>[5x]MSLINTKIKPFKNQAFKNGEFIEITEKDTEGRWSVFFFYPADFTFVCPTELGDVADHYEELQKLGVDVYAVSTDTHFTHKAWHSSSETIAKIKYAMIGDPTGALTRNFDNM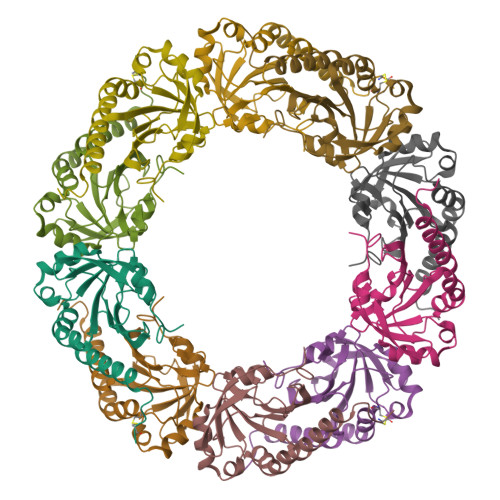REDEGLADRATFVVDPQGIIQAIEVTAEGIGRDASDLLRKIKAAQYVASHPGEVCPAKWKEGEATLAPSLDLVGKI> NVHNTKLASTSAENAIEKEQITTFHDVETPNRIDTPMAQDTSSARSMDDTHS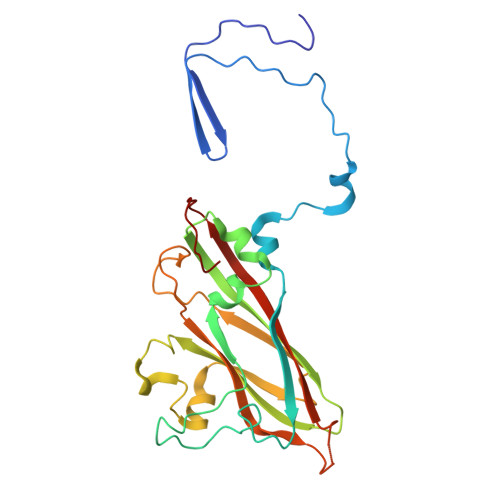IIQFLQRPVLIDNIEIVAGTTADNNTALSRYVLDRTNPQKYIKQWTLPSTVLKAGGKAQKLANFKYLRCDVQVKLVLNANPFIAGRLYLAYSPYDDKVAPERRIIYTSRAGVTGYPGVELDFQLDNSVEMTIPYASFQEAYDLVSGNEDFVQLYLFTIAPVLGPSAESANSKVDLSVYMWLDNISLVIPTYRLNPNL> MSWNHQSVEIAVRRTTVPSPNLPPGFDFTDPAIYAERLPVAEFAELRSAAPIWWNGQDPGKGGGFHDGGFWAITKLNDVKEISRHSDVFSSYENGVIPRFKNDIAREDIEVQRFVMLNMDAPHHTRLRKIISRGFTP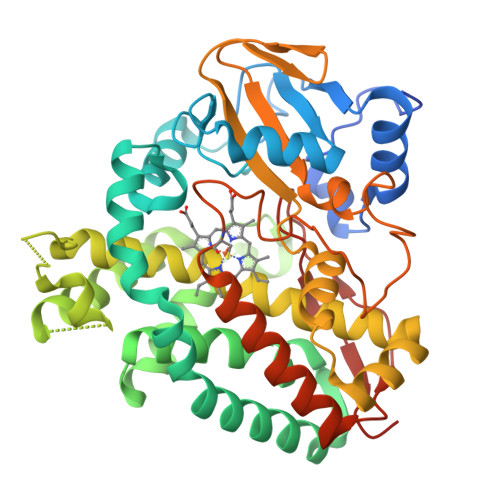RAVGRLHDELQERAQKIAAEAAAAGSGDFVEQVSCELPLQAIAGLLGVPQEDRGKLFHWSNEMTGNEDPEYAHIDPKASSAELIGYAMKMAEEKAKNPADDIVTQLIQADIDGEKLSDDEFGFFVVMLAVAGNETTRNSITQGMMAFAEHPDQWELYKKVRPETAADEIVRWATPVTAFQRTALRDYELSGVQIKKGQRVVMFYRSANFDEEVFQDPFTFNILRNPNPHVGFGGTGAHYCIGANLARMTINLIFNAVADHMPDLKPISAPERLRSGWLNGIKHWQVDYTGRCPVAH>MKFRIGELADKCGVNKETIRYYERLGLIPEPERTEKGYRMYSQQTVDRLHFIKRMQELGFTLNEIDKLLGVVDRDEAKCRDMYDFTILKIEDIQRKIEDLKRIERMLMDLKERCPENKDIYECPIIETLMKK[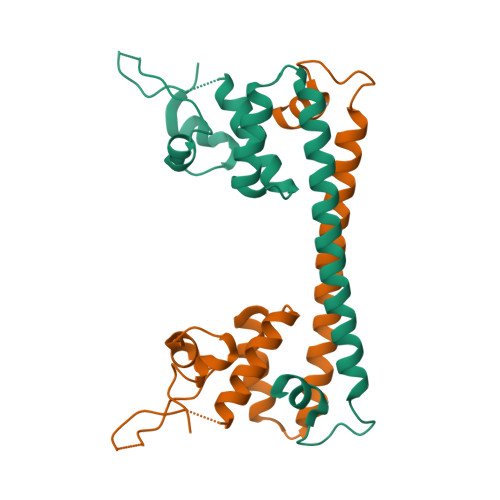2x]> VPDPRGIIINLDEGELCLNSAQCKSNCCQHDTILSLLRCALKARENSECSAFTLYGVYYKCPCERGLTCEGDKSLVGS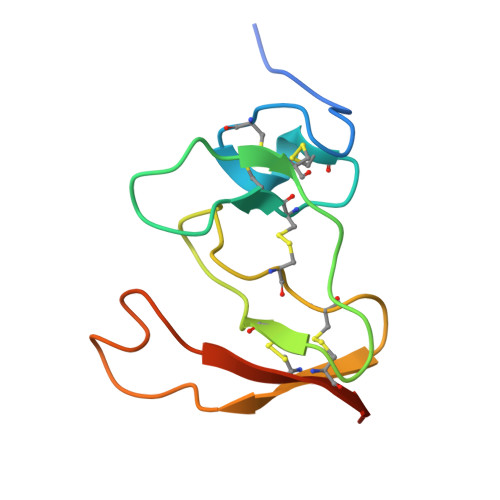ITNTNFGICHNVGRSDS> SNAMNHLPEKMRPYRDLLEKSAKEYVKLNVRKGKTGRYDSKIAGDPYFPKHETYPTDENGQPMKLLAQINFSHIPQLDGYPSSGILQFYISVHDDVYGLNFDDRCEQKNFRVIYFENIVENDDELVSDFSFIGTGECDFPILSEAAVEPVKSSEWVLPTDFQFEQYTGMETMEFFGQFGEDEEDIYNELAENGFGHKIGGYASFTQHDPREYAYKEHTIMLLQIDSDDDIDSMWGDV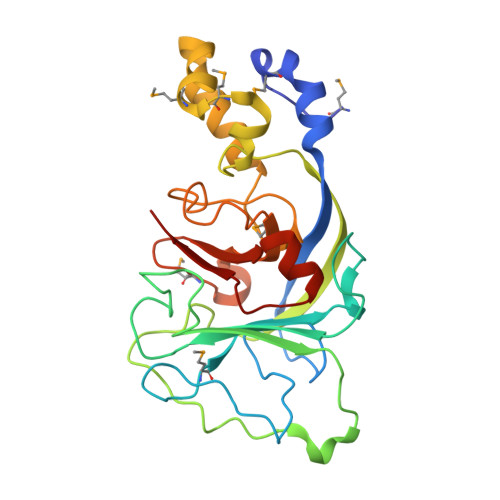GIANFFITPEDLRKKDFSNVLYNWDCS> KNTANIAKERLQNIVAERRRSDAEPHYLPQLRKDILEVICKYVQIDPEMVTV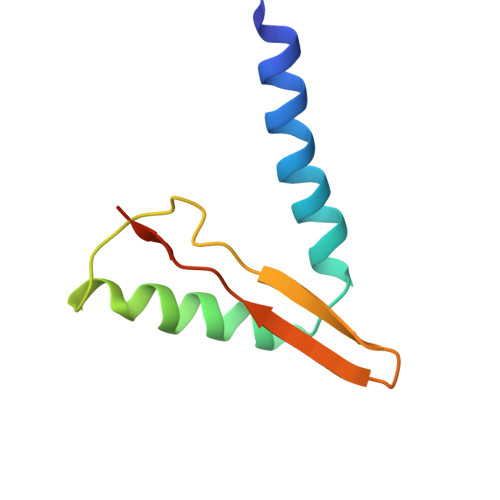QLEQKDGDISILELNVTLPEAEELK>MHHHHHHMTMDEQQPQAVT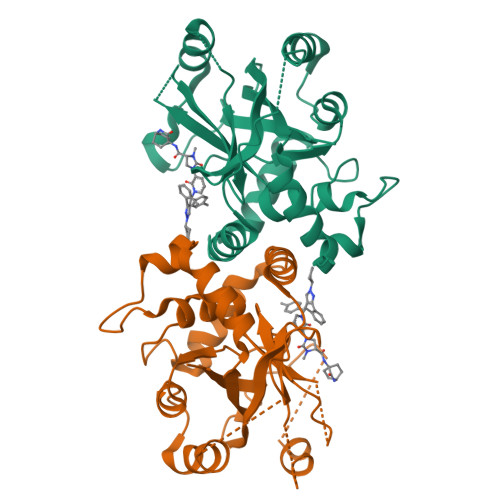PVYVGGFLARYDQSPDEAELLLPRDVVEHWLHAQGQGQPSLSVALPLNINHDDTAVVGHVAAMQSVRDGLFCLGCVTSPRFLEIVRRASEKSELVSRGPVSPLQPDKVVEFLSGSYAGLSLSSRRCDDVEQATSLSGSETTPFKHVALCSVGRRRGTLAVYGRDPEWVTQRFPDLTAADRDGLRAQWQRCGSTAVDASGDPFRSDSYGLLGNSVDALYIRERLPKLRYDKQLVGVTERESYVKA[2x]Bacteriophage Casadabanvirus JBD30, from the order Caudoviricetes, is a temperate phage that infects the bacterium Pseudomonas aeruginosa. The virion of bacteriophage JBD30 is composed of an icosahedral capsid, long flexible non-contractile tail, and a baseplate. Using its baseplate, JBD30 attaches to Pseudomonas aeruginosa via the bacterial type IV pilus, whose subsequent retraction brings the phage to the bacterial cell surface.

A pentamer of major capsid proteins on one of the capsid vertices is replaced by a connector complex formed by twelve copies of each portal (gp32) and adaptor (gp41) proteins and a hexamer of stopper proteins (gp42). The asymmetric reconstruction of the capsid–portal interface shows the symmetry mismatch between fivefold symmetry of the capsid and twelvefold symmetry of the portal. The portal complex is surrounded by five hexamers of major capsid proteins. Two major capsid proteins from each of the hexamers contact the portal. One of the major capsid proteins binds the portal complex with its extended loop and peripheral domain. The second major capsid protein, which is positioned counterclockwise when looking at the portal from the inside of the capsid, contacts the portal with its peripheral domain. In contrast, at the interface with the portal complex the N-terminus of the major capsid protein (residues 2–14) turns back and forms a short α-helix positioned parallel to the extended loop of the neighbouring major capsid protein, thus leaving more space around the fivefold axis for the portal complex. The reduction of symmetry from the twelvefold of the connector to the sixfold of the tail occurs at the adaptor–stopper interface. Asymmetric reconstruction of the JBD30 virion connector complex contains double-stranded DNA passing through the portal channel. The DNA does not interact with the stopper proteins and continues uninterrupted into the tail discs.

>[420x]MARQNSAAKTTAKSKTDPATEKPKDDTLPDSTDDASPTAPETPATKPDSASDEVEGVFVRATVERRCRAGFCFDKEGQGFADGVLSDEQLEALESDPLLKVERCTFSGNQEGE;>[415x]MAIITPALISALKTSFQKHFQDALATAPSTYLQVATVIPSTTASNTYGWLGQFPKLREWIGQRVIKDMAAQGYQITNKLFESTVGVKRTDIEDDNLGVYGPLMQEMGRAAGAHPDELVFALLKAGNANLCYDGQNFFDTDHPVYPNVDGTGTATTVSNLFAPAADPGAAWYLLDTSRSLKPLIYQERMKPSFTSMTKEDDEQVFMADEYRYGVRSRCNVGFGFWQLAAMSTEELNQVNFEKVYDAMRNQKADGGRPLDIRPNLLVVPTTLRSKAKEVVGVQRLANGADNPNFELVQVLDTAWLN;>[12x]MSYCTLADLIEQYSEQKIREVSDRVNKPATTIDTVIVDRAIADADSEIDLHLHGRYQLPLASVPTALKRIACGLAYANLHIVLKEENPVYKTAEHLRKLLSGIANGKLSLALDADGKPAPVANTVQISEGRNDWGADW;>MAQIVDVYGNPIRTQQLREPQTSRLAGLAKEFAQHPAKGLTPAKLARILVEAEQGNLQAQAELFMDMEERDAHLFAEMSKRKRAILGLDWAVEPPRNASAAEKADADYLHELLLDLEGLEDLLLDALDGIGHGYSCIELEWALQGREWMPLAFHHRPQSWFQLNPEDQNELRLRDNSPAGEALQPFGWIIHRPRARSGYVARSGLFRVLAWPYLFRHYATSDLAEMLEIYGLPIRLGKYPPGTADEEKATLLRAVTGLGHAAAGIIPETMAIDFQQAAQGSSDPFLAMMRQSEDAISKAVLGGTLTSTTSQSGGGAFALGQVHNEVRHDLLASDARQLAATLSRDLLWPLLVLNRPGSPDVRRAPRLVFDLREQADITSMAQSIPALVNVGLEIPSAWVYDKLGIPQPAKNEPVLRSAAQPAILSRQHGQRVAALATIVGPRYGDQQALDKALASLPAKDMQDQVNDLLAPLLEAVNRGDSETELLGALAEAFPDMDDSALTDALHRLLFAADTWGRLHGNLDRID[12x];>MSDPFDYLFLEPLLIERIRSEVPGLAIVSGVPDLATLSEQDQPAPSAYVVYLGDETGTGADHQGGQRAIQTVGQQWAVVLVVHYADSSNSGEGARREAGPLLGRLVKALTGWAPAIDVAPLARSARQSPATYASGYLYFPLVFTARFVYPRIKSWKP[6x];>MAQETYFYGQGEIDAAPIVNGVLGKWRWIQDVSAMSIQLAVEKVEHKESYSGQKALVRSFPIGKTATVNITLHSIGPDNLALTLYGKVVAKAAGSVTGEVLPADLVAGDVIRLANFGVSELVITDSASSPAPLDPQYYALRADGAYGEVQLLGLPTPAPTQPFKAAYEYAATKQVGMFTAPQPTVALRYKGINLAEGGAPVIVELYKVATDPLQELALISDGNTVAGMQISGGILLDTSKPDTGDLGRFGRIIQLG[6x]> LYGPGDEDPNPKHPKTPDKCDPSLSLDAITSLRGETMIFKDRFFWRLHPQQVDAELFLTKSFWPELPNRIDAAYEHPSHDLIFIFRGRKFW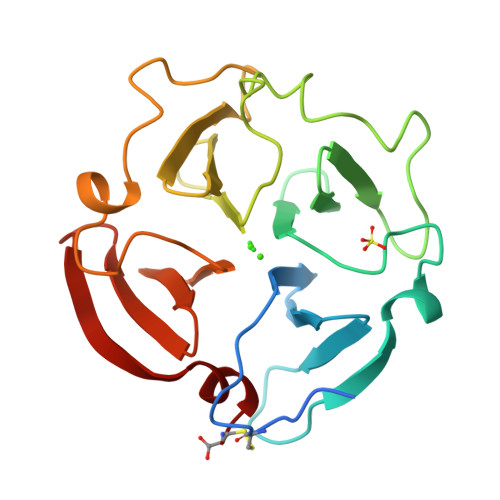ALNGYDILEGYPKKISELGLPKEVKKISAAVHFEDTGKTLLFSGNQVWRYDDTNHIMDKDYPRLIEEDFPGIGDKVDAVYEKNGYIYFFNGPIQFEYSIWSNRIVRVMPANSILWC> MTSFYKITAYNSQALYFWGTDADVDRYVDWLNRDREINVYAAEAIPEAEWAQYEGRDDVLSGEECGWDDF;>TIEKRYDFVFLFDVQDGNPNGDPDAGNLPRIDPQTGEGLVTDVCLKRKVRNFIQMTQNDEHHDIFIREKGILNNLIDEAHEQENVKGKEKGEKTEAARQYMCSRYYDIRTFGAVMTTGKNAGQVRGPVQLTFSRSIDPIMTLEHSITRMAVTNEKDASETGDNRTMGRKFTVPYGLYRCHGFISTHFAKQTGFSENDLELFWQALVNMFDHDHSAARGQMNARGLYVFEHSNNLGDAPADSLFKRIQVVKKDGVEVVRSFDDYLVSVDDKNLEETKLLRKLGG[7x];>GLDRNRQDIGYVLGRLFAVLEKIQAEANPGLNATIADRYFGSASSTPIAVFGTLMRLLPHHLNKLEFEGRAVQLQWEIRQILEHCQRFPNHLNLEQQGLFAIGYYHETQFLFTKDALKNLFNEA[4x];> MILHALTQYYQRKAESDGGIAQEGFENKEIPFIIVIDKQGNFIQLEDTRELKVKKKVGRTFLVPKGLGRSGSKSYEVSNLLWDHYGYVLAYAGEKGQEQADKQHASFTAKVNELKQALPDDAGVTAVAAFLSSAEEKSKVMQAANWAECAKVKGCNLSFRLVDEAVDLVCQSKAVREYVSQANQTQSDNAQKGICLVTGKAAPIARLHNAVKGVNAKPAPFASVNLSAFESYGKEQGFAFPIGEQAMFEYTTALNTLLAGENRFRIGDVTTVCWGAKRTPLEESLASMINGGGKDKPDEHIDAVKTLYKSLYNGQYQKPDGKEKFYLLGLSPNSARIVVRFWHETTVAALSESIAAWYDDLQMVRGENSPYPEYMPLPRLLGNLVLDGKMENLPSDLIAQITDAALNNRVLPVSLLQAALRRNKAEQKITYGRASLLKAYINRAIRAGRLKNMKELTMGLDRNRQDIGYVLGRLFAVLEKIQAEANPGLNATIADRYFGSASSTPIAVFGTLMRLLPHHLNKLEFEGRAVQLQWEIRQILEHCQRFPNHLNLEQQGLFAIGYYHETQFLFTKDALKNLFNEA;> RFILEISGDLACFTRSELKVERVSYPVITPSAARNILMAILWKPAIRWKVLKIEILKPIQWTNIRRNEVGTKMSERSGSL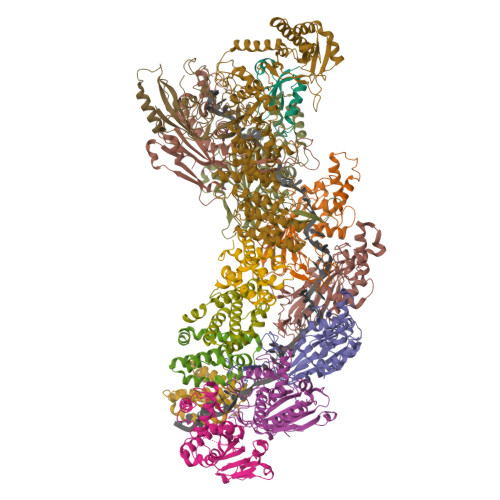YIEDNRQQRASMLLKDVAYRIHADFDMTSEAGESDNYVKFAEMFKRRAKKGQYFHQPYLGCREFPCDFRLLEKAEDGLPLEDITQDFGFMLYDMDFSKSDPRDSNNAEPMFYQCKAVNGVITVPP>SNAMSGFLEQRLGHCLRQMAEKGLEALLVTHLTNSYYLTGFSGTAATVL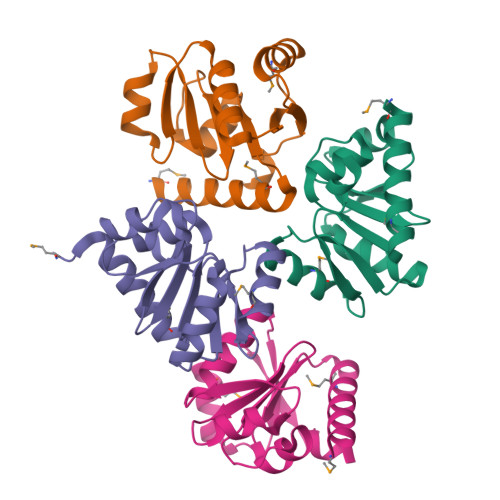ITAKRRVLITDSRYTLLAKASVEGFDIIESRTPLKVVAELLEADQIDCLGFEDQVSFSFYQAMQAELSGITLLAQSGFVEHLR[4x]> MTDVDKRKIKIILNGEMEEAELHMITSPNRHCCLKIFHNNNQLAESNDTDYFSCFADLRNQLKNIIFLCKGAKINVYPSAMSRDMSDGIVAYETTLGQPGLPENQVHIFDF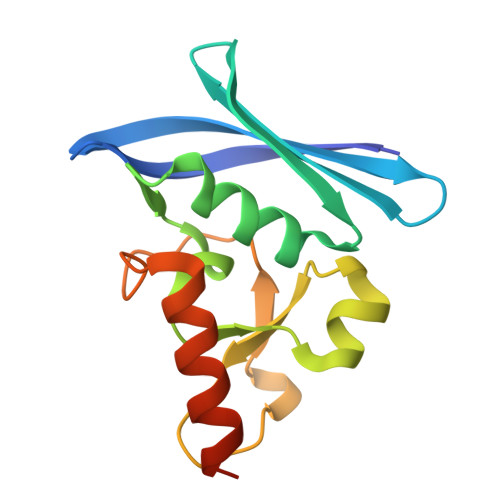EDKYVDITPEEQRKFHSQWFESLVDHHHHHH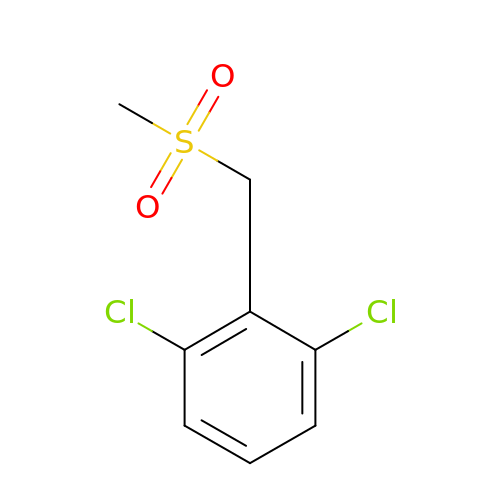1,3-dichloro-2-[(methylsulfonyl)methyl]benzene | C8 H8 Cl2 O2 S | YQGFLUVOLNGRET-UHFFFAOYSA-N> NVPELIGAQAHAVNVILDAETAYPNLIFSDDLKSVRLGNKWERLPDGPQRFDSCIIVLGSPSFLSGRRYWEVEVGDKTAWILGACKTS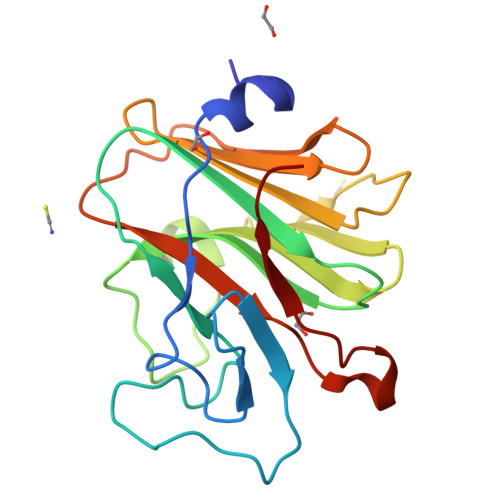ISRKGNMTLSPENGYWVVIMMKENEYQASSVPPTRLLIKEPPKRVGIFVDYRVGSISFYNVTARSHIYTFASCSFSGPLQPIFSPGTRDGGKNTAPLTICPVG3-methyl-5-[5-(1-methylethyl)-1H-benzimidazol-2-yl]-N-(1-methylpiperidin-4-yl)-1H-pyrazole-4-carboxamide | C21 H28 N6 O | 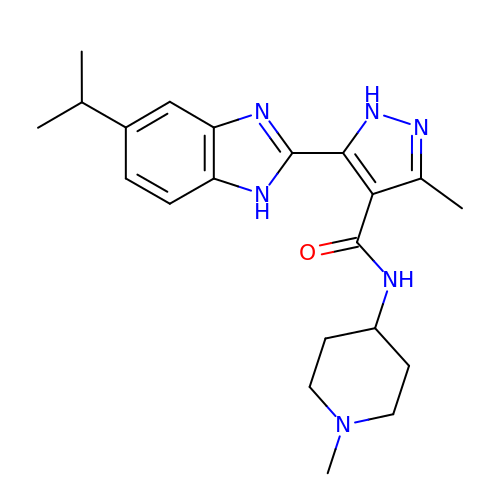PFGGMNGDLVJXNC-UHFFFAOYSA-N3-[(4S)-2,5-DIOXOIMIDAZOLIDIN-4-YL]PROPANOIC 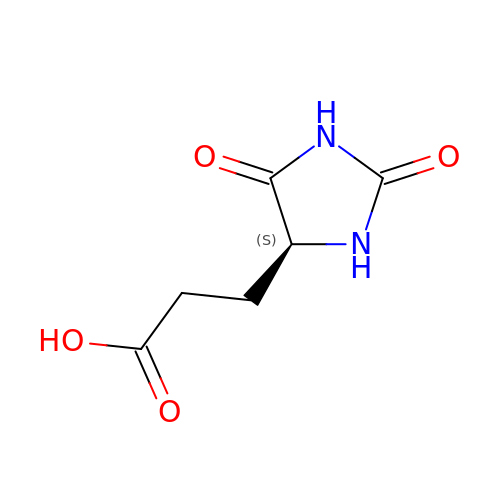ACID | C6 H8 N2 O4 | VWFWNXQAMGDPGG-VKHMYHEASA-N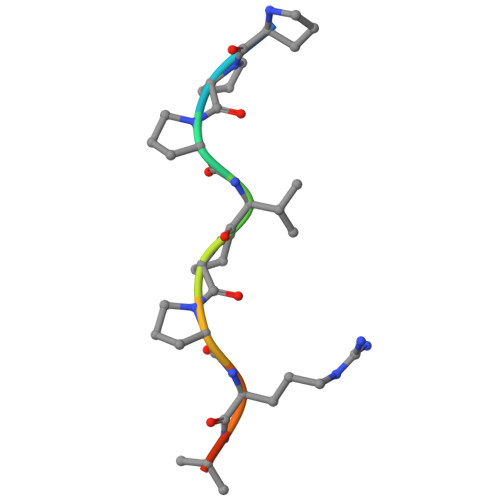> PPPVPPRRRR> MNVIAILNHMGVYFKEEPIRELHRALERLNFQIVYPNDRDDLLKLIENNARLCGVIFDWDKYNLELCEEISKMNENLPLYAFANTYSTLDVSLNDLRLQISFFEYALGAAEDIANKIKQTTDEYINTILPPLTKALFKYVREGKYTFCTPGHMGGTAFQKSPVGSLFYDFFGPNTMKSDISISVSELGSLLDHSGPHKEAEQYIARVFNADRSYMVTNGTSTANKIVGMYSAPAGSTILIDRNCHKSLTHLMMMSDVTPIYFRPTRNAYGILGGIPQSEFQHATIAKRVKETPNATWPVHAVITNSTYDGLLYNTDFIKKTLDVKSIHFDSAWVPYTNFSPIYEGKCGMSGGRVEGKVIYETQSTHKLLAAFSQASMIHVKGDVNEETFNEAYMMHTTTSPHYGIVASTETAAAMMKGNAGKRLINGSIERAIKFRKEIKRLRTESDGWFFDVWQPDHIDTTECWPLRSDSTWHGFKNIDNEHMYLDPIKVTLLTPGMEKDGTMSDFGIPASIVAKYLDEHGIVVEKTGPYNLLFLFSIGIDKTKALSLLRALTDFKRAFDLNLRVKNMLPSLYREDPEFYENMRIQELAQNIHKLIVHHNLPDLMYRAFEVLPTMVMTP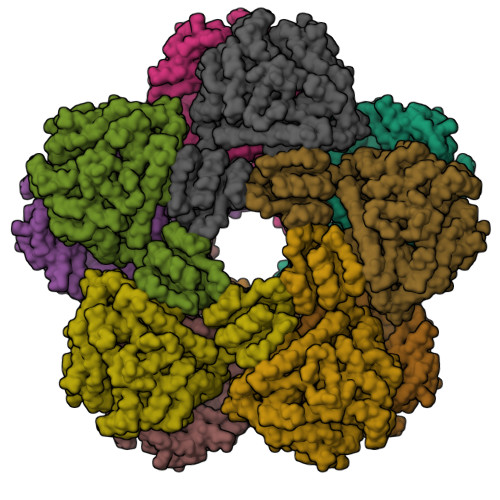YAAFQKELHGMTEEVYLDEMVGRINANMILPYPPGVPLVMPGEMITEESRPVLEFLQMLCEIGAHYPGFETDIHGAYRQADGRYTVKVLKE> MHTAEFLETEPTEISSVLAGGYNHPLLRQWQSERQLTKNMLIFPLFISDNPDDFTEIDSLPNINRIGVNRLKDYLKPLVAKGLRSVILFGVPLIPGTKDPVGTAADDPAGPVIQGIKFIREKFPELYIICDVCLCEYTSHGHCGVLYDDGTINRERSVSRLAAVAVNYAKAGAHCVAPSDMIDGRIRDIKRGLINANLAHKTFVLSYAAKFSGNLYGPFRDAACSAPSNGDRKCYQLPPAGRGLARRAL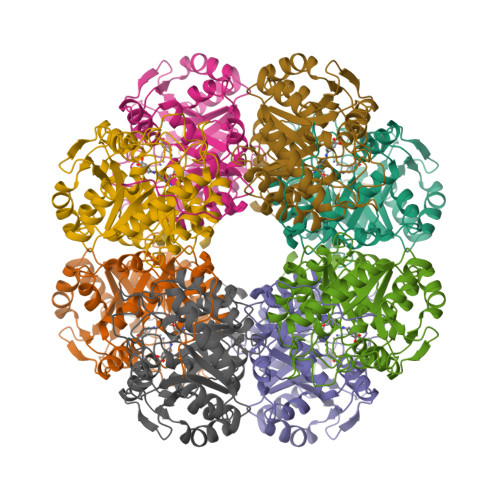ERDMSEGADGIIVKPSTFYLDIMRDASEICKDLPICAYHVSGEYAMLHAAAEKGVVDLKTIAFESHTGFLRAGARLIITYLAPEFLDWLDEEN> GPHMATGQDRVVALVDMDCFFVQVEQRQNPHLRNKPCAVVQYKSWKGGGIIAVSYEARAFGVTMSMWADDAKKLCPDLLLAQVRESRGKANLTKYREASVEVMEIMSRFAVIERASIDEAYVDLTSAVQERLQKLQGQPISADLLPSTYIEGLPQGPTTAEETVQKEGMRKQGLFQWLDSLQIDNLTSPDLQLTVGAVIVEEMRAAIERETG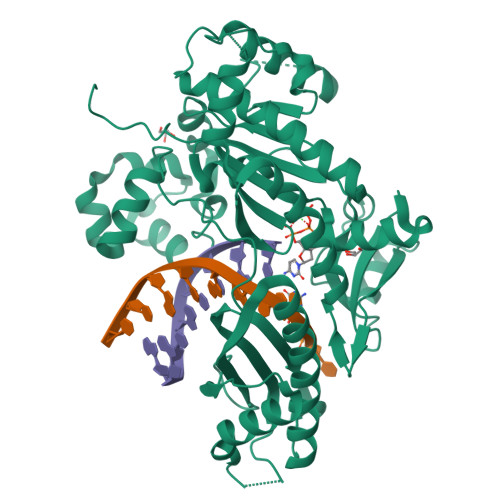FQCSAGISHNKVLAKLACGLNKPNRQTLVSHGSVPQLFSQMPIRKIRSLGGKLGASVIEILGIEYMGELTQFTESQLQSHFGEKNGSWLYAMCRGIEHDPVKPRQLPKTIGCSKNFPGKTALATREQVQWWLLQLAQELEERLTKDRNDNDRVATQLVVSIRVQGDKRLSSLRRCCALTRYDAHKMSHDAFTVIKNCNTSGIQTEWSPPLTMLFLCATKFSAS> MGAQVSSQKVGAHENSNRAYGGSTINYTTINYYKDSASNAASKQDYSQ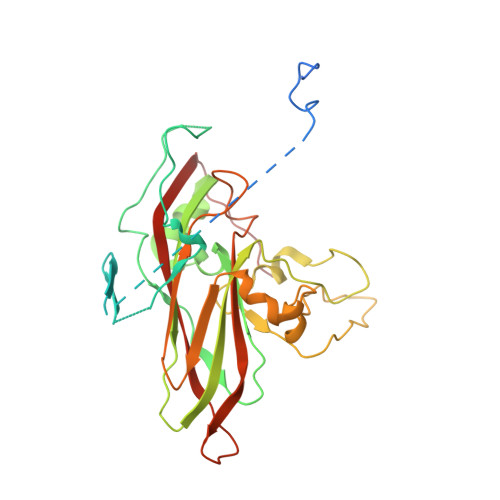DPSKFTEPLKDVLIKTAPALNSPNVEACGYSDRVLQLTIGNSTITTQEAANSVVAYGRWPEFIRDDEANPVDQPTEPDVATCRFYTLDTVMWGKESKGWWWKLPDALRDMGLFGQNMYYHYLGRSGYTVHVQCNASKFHQGALGVFAIPEYCLAGDSDKQRYTSYANANPGEKGGKFYSQFNRDTAVTSPKREFCPVDYLLGCGVLLGNAFVYPHQIINLRTNNSATIVLPYVNAMAIDSMVKHNNWGIAILPLSPLDFAQESSVEIPITVTIAPMCSEFNGLRNVTAPKFQ>[2x]SNAMKKFSVVIAGGGSTFTPGIVLMLLANQDRFPLRSLKFYDNDGARQETIAEACKVILKEQAPEIEFSYTTDPQAAFTDVDFVMAHIRVGKYPMREQDEKIPLRHGVLGQETCGPGGIAYGMRSIGGVLELVDYMEKYSPNAWMLNYSNPAAIVAEATRRLRPNAKILNICDMPIGIEGRMAQIVGLKDRKQ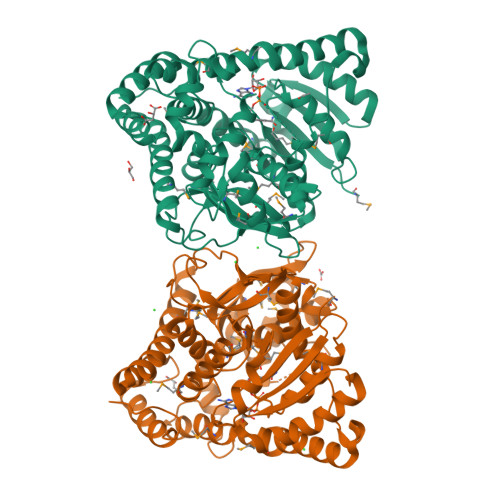MRVRYYGLNHFGWWTSIEDLDGNDLMPKLREYVAKYGYVPPSNDPHTEASWNDTFAKAKDVQALDPQTMPNTYLKYYLFPDYVVAHSNPERTRANEVMDHREKNVFSACRAIIAAGKSTAGDLEIDEHASYIVDLATAIAFNTQERMLLIVPNNGAIHNFDADAMVEIPCLVGHNGPEPLTVGDIPHFQKGLMSQQVAVEKLVVDAWEQRSYHKLWQAITLSKTVPSASVAKAILDDLIAANKDYWPELH> MQSINFRTARGNLSEVMNNVEAGEEVEITRRGREPAVIASKATFE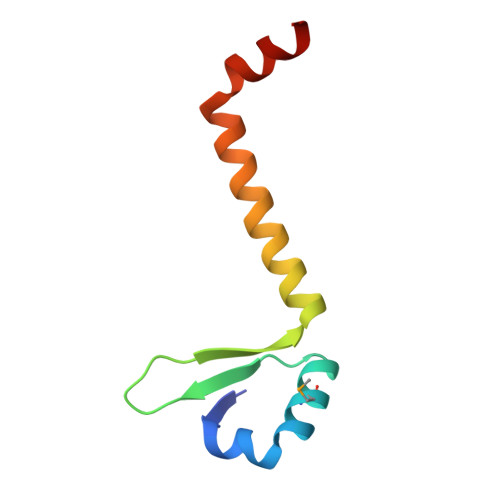AYKKAALDAEFASLFDTLDSTNKELVNR>MRRSVYFCGSIRGGREDQALYARIVSRLRRYGKVLTEHVADAELEPLGEEAAGGDQFIHEQNLNWLQQADVVVAEVTQPSLGVGYELGRAVALGKPILCLFRPQSGRVLSAMIRGAADGSRFQVWDY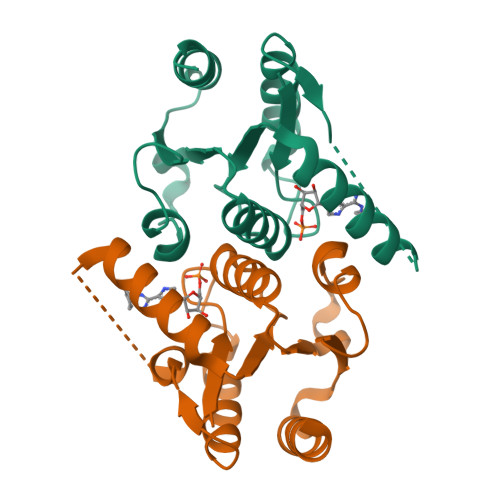AEGEVETMLDRYFEAYLVEHHHHHH[4x]>MRKEAIHHRSTDNFAYAYDSETLHLRLQTKKNDVDHVELLFGDPYEWHDGAWQFQTMPMRKTGSDGLFDYWLAEVKPPYRRLRYGFVLRAGGEKLVYTEKGFYHEAPSDDTAYYFCFPFLHRVDLFQAPDWVKDTVWYQIFPERFANGNPAISPKGARPWGSEDPTPTSFFGGDLQGIIDHLDYLADLGITGIYLTPIFRAPSNHKYDTADYFEIDPHFGDKETLKTLVKRCHEK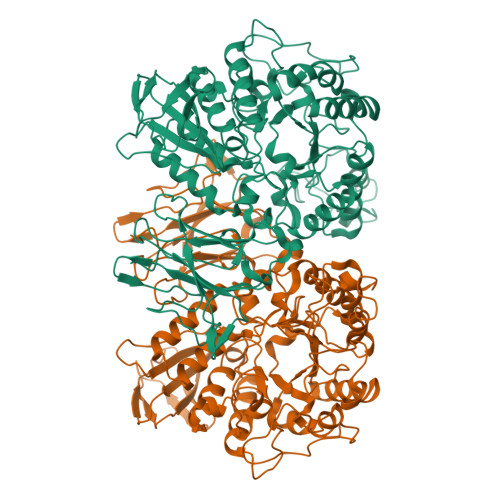GIRVMLDAVFNHCGYEFAPFQDVLKNGAASRYKDWFHIREFPLQTEPRPNYDTFAFVPHMPKLNTAHPEVKRYLLDVATYWIREFDIDGWRLDVANEIDHQFWREFRQAVKALKPDVYILGEIWHDAMPWLRGDQFDAVMNYPLADAALRFFAKEDMSASEFADRLMHVLHSYPKQVNEAAFNLLGSHDTPRLLTVCGGDVRKVKLLFLFQLTFTGSPCIYYGDEIGMTGGNDPECRKCMVWDPEKQNKELYEHVKQLIALRKQYRALRRGDVAFLTADDEVNHLVYAKTDGNETVMIIINRSNEAAEIPMPIDARGKWLVNLLTGERFAAEAETLCVSLPPYGFVLYAVESW[2x]> HHHHHHSSGLVPRGSHMRIVSAGSAVTELILALGAEQQLVAVDVTSEVPSSLNLPTVGYHRRLAAEGLLTLEPTHLIGSDEMGPDTALQQLRSSGIQVNVINSDSTPQGLLTRIDQIAQITHTEQHAQKLKENVQQQINALQAKRPEKPKKVLFLLLHEGRAANVAGSDTVPDTIIGLIGAHNPASPSITSYKPLSMESMIEMQPDMVLVSGRSLEKLGGADAVLNAVPMLAATPA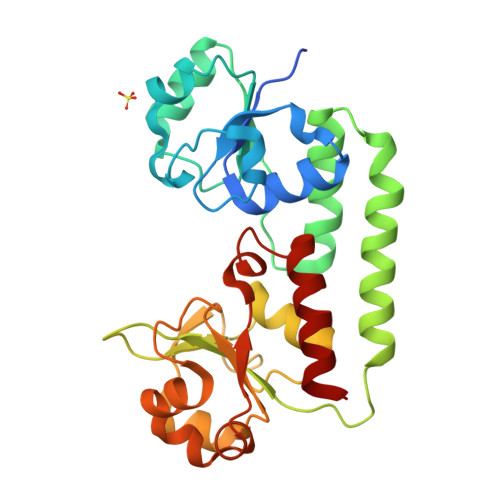GQNKNIVAIDGHALVGGLGLKSLQEAQRIQTLLYP>[2x]MHHHHHHSSGRENLYFQGPTESMESHQYQTEVTRLMDIIVNSLYTQKEVFLRELISNAADALEKIRFLSLSDESVLGEEKKLEIRISANKEKNILSITDTGIGMTKVDLINNLGTIAKSGTSNFLEAISKSGGDMSLIGQFGVGFYSAF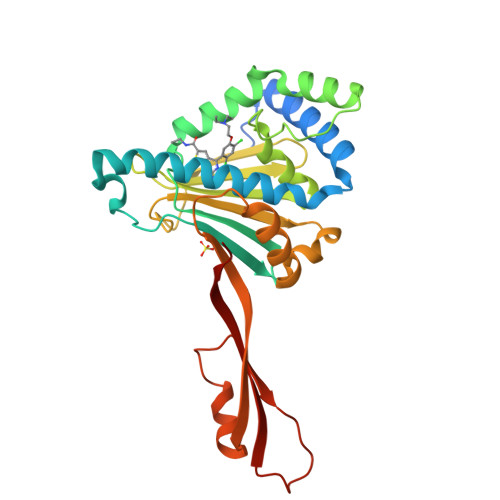LVADKVIVYTKNNDDEQYIWESTADAKFTIYKDPRGATLKRGTRISLHLKEDATNLLNDKKLMDLISKYSQFIQFPIYLLHENVYTEEVLADIAKDMVNDPNYDSVKVEETDDPNKKTRTVEKKVKKWTLMN>[2x]MELRHLRYFVAVVEEQSFTKAADKLCIAQPPL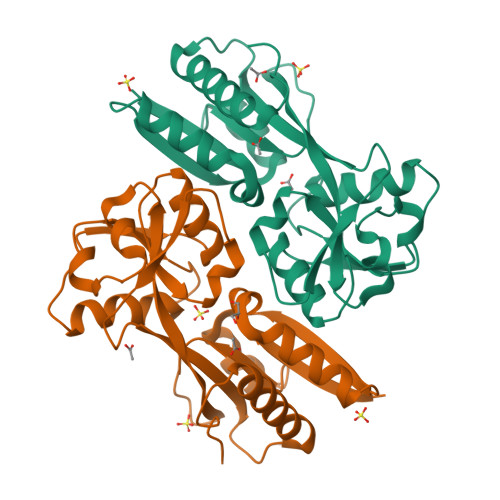SRQIQNLEEELGIQLLERGSRPVKTTPEGHFFYQYAIKLLSNVDQMVSMTKRIASVEKTIRIGFVGSLLFGLLPRIIHLYRQAHPNLRIELYEMGTKAQTEALKEGRIDAGFGRLKISDPAIKHSLLRNERLMVAVHASHPLNQMKDKGVHLNDLIDEKILLYPSSPKPNFSTHVMNIFSDHGLEPTKINEVREVQLALGLVAAGEGISLVPASTQSIQLFNLSYVPLLDPDAITPIYIAVRNMEESTYIYSLYETIRQIYAYEGFTEPPNWLEHHHHHH>[2x]GMACGLVASNLNLKPGECLRVRGEVAPDAKSFVLNLGKDSNNLCLHFNPRFNAHGDANTIVCNSKDGGAWGTEQREAVFPFQPGSVAEVCITFDQANLTVKLPDGYEFKFPNRL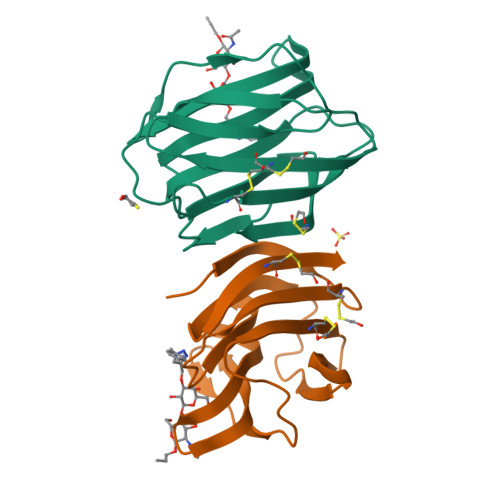NLEAINYMAADGDFKIKCVAFD(12E)-10-oxooctadec-12-enoic 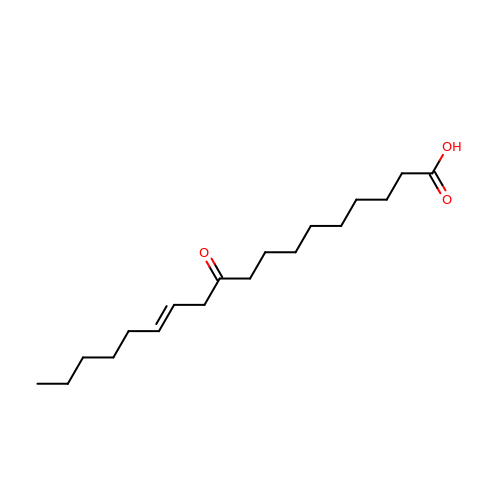acid | C18 H32 O3 | IEQLMTRAAYQDSD-DHZHZOJOSA-N> ATCDDGRTTANAACCILFPILDDIQENLFDGANCGEEVHESLRLTFHDAIGFSPTLGGGGADGSIIAFDTIETNFPANAGIDEIVSAQKPFVAKHNISAGDFIQFAGAVGVSNCPGGVRIPFFLGRPDAVAASPDHLVPEPFDSVDSILARMGDAGFSPVEVVWLLASHSIAAADKVDPSIPGTPFDSTPEVFDSQFFIETQLKGRLFPGTADNKG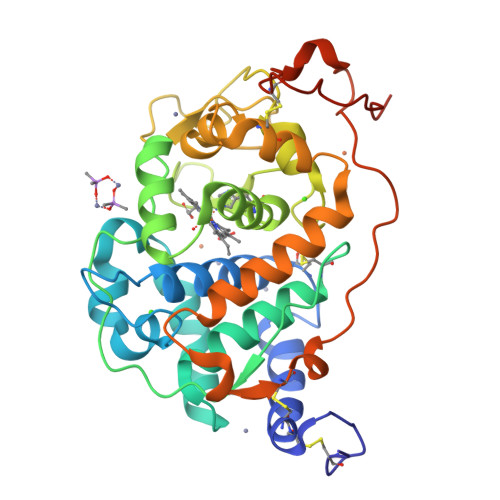EAQSPLQGEIRLQSDHLLARDPQTACEWQSMVNNQPKIQNRFAATMSKMALLGQDKTKLIDCSDVIPTPPALVGAAHLPAGFSLSDVEQACAATPFPALTADPGPVTSVPPVPGS>[6x]GHMGKPDISAKDLRNIMYDHLPGFGTAFHQLVQVICKLGKDSNSLDIIHAEFQASLAEGDSPQCALIQITKRVPIFQDAAPPVIHIRSRGD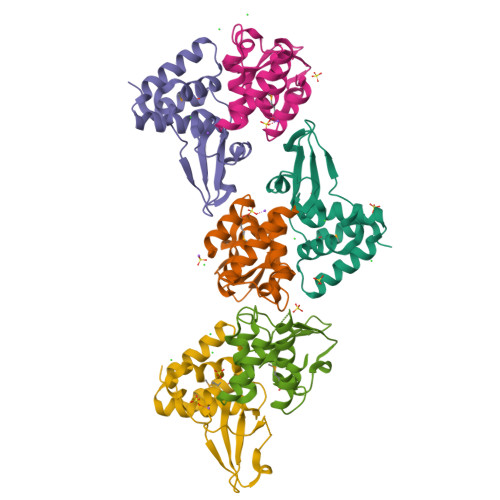IPRACQKSLRPVPPSPKIDRGWVCVFQLQDGKTLGLAI> TIARTIVLQESIGKGRFGEVWRGKWRGEEVAVKIFSSREERSWFREAEIYQTVMLRHENILGFIAADNKDNGTWTQLWLVSDYHEHGSLFDYLNRYTVTVEGMIKLALSTASGLAHLHMEIVGTQGKPAIAHRDLKSKNILVKKNGTCCIADLGLAVRHDSATDTIDIAPNHRVGTKRYMAPEVLDDSINMKHFESFKRADIYAMGLVFWEIARRCSIGGIHEDY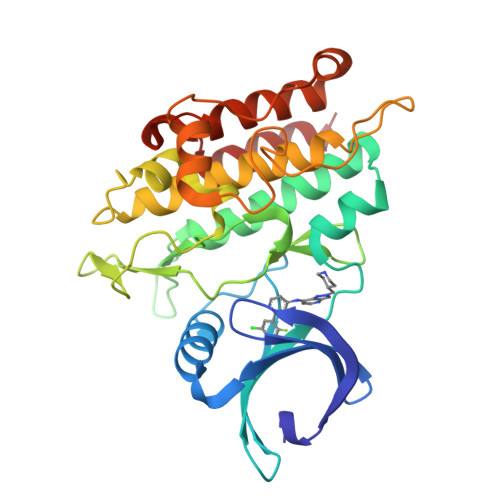QLPYYDLVPSDPSVEEMRKVVCEQKLRPNIPNRWQSCEALRVMAKIMRECWYANGAARLTALRIKKTLSQLSQQ> GAMDKQKPRYEIRWRVIESISPDGHEYIYVDPMQLPYDSRWEFPRDGLVLGRVLGSGAFGKVVEGTAYGLSRSQPVMKVAVKMLKPTAR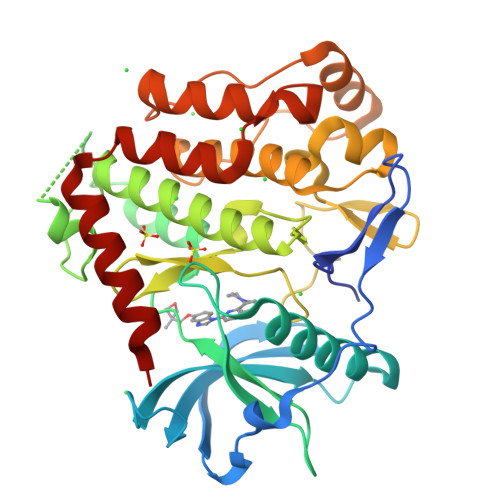SSEKQALMSELKIMTHLGPHLNIVNLLGACTKSGPIYIITEYCFYGDLVNYLHKNRDSFLSHKKKSMLDSEVKNLLSDDNSEGLTLLDLLSFTYQVARGMEFLASKNCVHRDLAARNVLLAQGKIVKICDFGLARDIMHDSNYVSKGSTFLPVKWMAPESIFDNLYTTLSDVWSYGILLWEIFSLGGTPYPGMMVDSTFYNKIKSGYRMAKPDHATSEVYEIMVKCWNSEPEKRPSFYHLSEIVENLLPGQYKKSYEKIHLDFLKSD6-chloroguanine | C5 H4 Cl N5 | 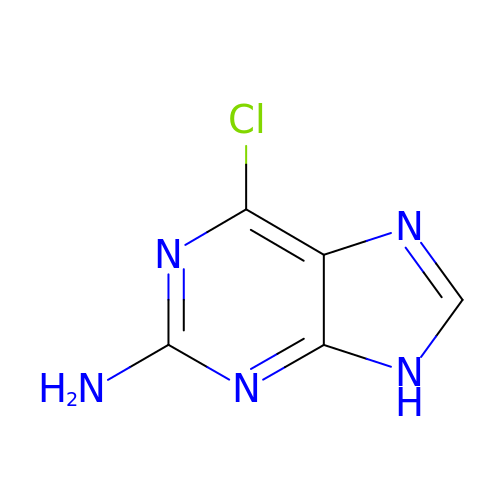RYYIULNRIVUMTQ-UHFFFAOYSA-N>[3x]MKKLTIGLIGNPNSGKTTLFNQLTGSRQRVGNWAGVTVERKEGQFSTTDHQVTLVDLPGTYSLTTISSQTSLDEQIACHYILSGDADLLINVVDASNLERNLYLTLQLLELGIPCIVALNMLDIAEKQNIRIEIDALSARLGCPVIPLVATRGRGIEALKLAIDRYKANENVELVHYAQPLLNEADSLAKVMPSDIPLKQRRWLGLQML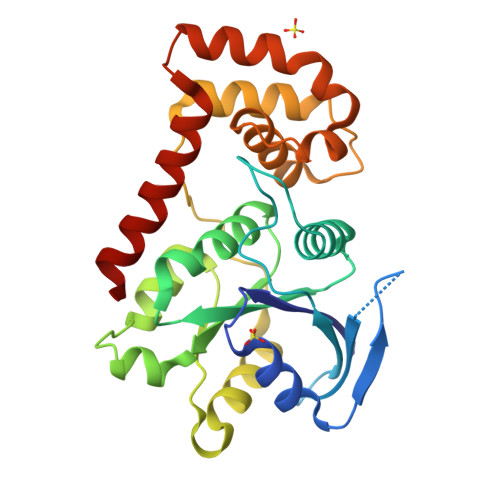EGDIYSRAYAGEASQHLDAALARLRNEMDDPALHIADARYQCIAAICDVVSN>[4x]SSLSRAVLDGASAAEIEAAPVPDTYLALHLRAEDADMFKGVADKDVRKSLRLGEVPMPELAPDEVLVAVMASSINYNTVWSAMFEPIPTFHFLKQNARQGGWATRHDQPYHVLGSDCSGVVVRTGIGVRRWKPGDHVIVHPAHVDEQEPATHGDGMLGTEQRAWGFETNFGGLAEYGVVRASQLLPKPAHLTWEEAAVSPLCAGTAYRMLVSDRG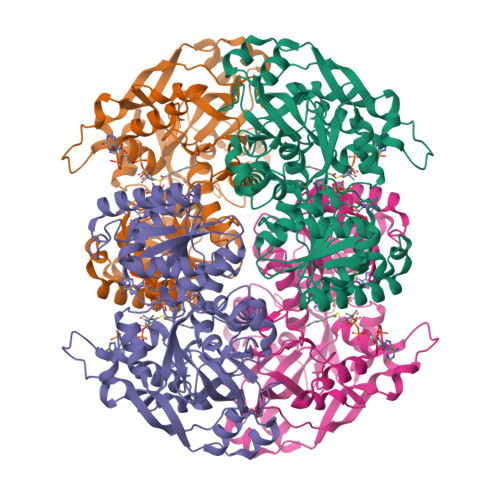AQMKQGDIVLIWGASGGLGSYAIQFVKNGGGIPVAVVSSAQKEAAVRALGCDLVINRAELGITDDIADDPRRVVETGRKLAKLVVEKAGREPDIVFEHTGRVTFGLSVIVARRGGTVVTCGSSSGYLHTFDNRYLWMKLKKIVGSHGANHEEQQATNRLFESGAVVPAMSAVYPLAEAAEACRVVQTSRQVGKVAVLCMAPEQGLGVTDPDLRARLGEDRLNPLRGLTATSR> MGSSHHHHHHSSGPQQGLRKGDIKIKIVSGTASSFQSGSNIEKSFDGDYSTLYHSSWSNGASNYFPITLTYNFETVTDVDYLIYHPRNN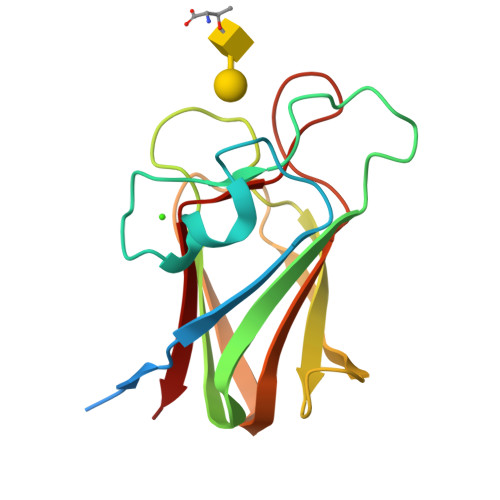GNNGRFKETEIQYSADGHTFTKLIDKDFQGSATAGKVTFDQTIQAKSFRFIVKSGSGDGQGFASCAEMEFFAK>[2x]GSMETSMPEYYEVFGEFRGVLMDKRFTKYWEDVEMFLARPDDLVIATYPKSGTTWISEVVYMIYKEGDVEKCKEDAIFNRIPYLECRNEDLINGIKQLKEKESPRIVKTHLPPKLLPASFWEKNCKMIYLCRNAKDVAVSYYYFLLMITSYPNPKSFSEFVEKFMQGQVPYGSWYDHVKAWWEKSKNSRVLFMFYEDMKEDIRREVVKLIEFLERKPSAELV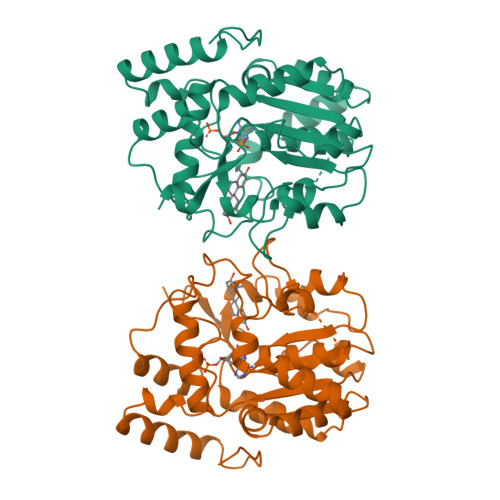DRIIQHTSFQEMKNNPSTNYTMMPEEMMNQKVSPFMRKGIIGDWKNHFPEALRERFDEHYKQQMKDCTVKFRMEL4-{(2S)-2-[2-(4-chlorophenyl)-5,6-difluoro-1H-benzimidazol-1-yl]-2-cyclohexylethoxy}-3-fluorobenzoic acid | 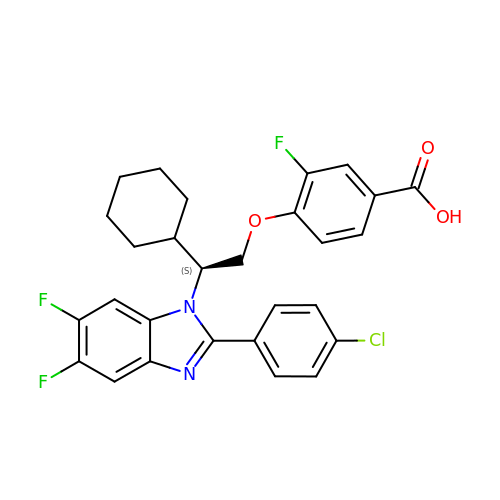C28 H24 Cl F3 N2 O3 | CPOSGAZIIDJVMJ-RUZDIDTESA-N>[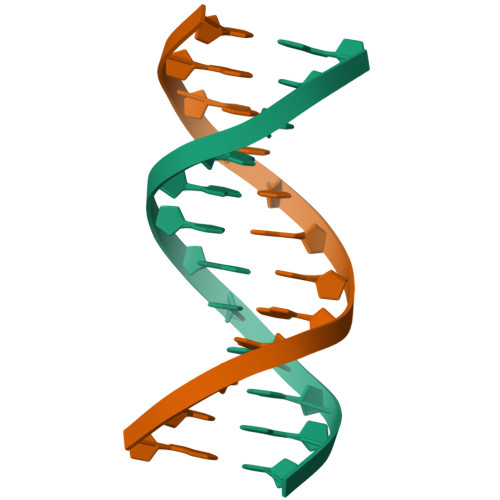2x]ACCGGTACCGGT> MSHPDYRMNLRPLGTPRGVSAVAGPHDIGASPGDKKSKNRSTRGKKKSIFETYMSKEDVSEGLKRGTLIQGVLRINPKKFHEAFIPSPDGDRDIFIDGVVARNRALNGDLVVVKLLPEEHWKVVKPESNDKETEAAYESDIPEELCGHHLPQQSLKSYNDSPDVIVEAQFDGSDSEDGHGITQNVLVDGVKKLSVCVSEKGREDGDAPVTKDETTCISQDTRALSEKSLQRSAKVVYILEKKHSRAATGFLKLLADKNSELFRKYALFSPSDHRVPRIYVPLKDCPQDFVARPKDYANTLFICRIVDWKEDCNFALGQLAKSLGQAGEIEPETEGILTEYGVDFSDFSSEVLECLPQGLPWTIPPEEFSKRRDLRKDCIFTIDPSTARDLDDALSCKPLADGNFKVGVHIADVSYFVPEGSDLDKVAAERATSVYLVQKVVPMLPRLLCEELCSLNPMSDKLTFSVIWTLTPEGKILDEWFGRTIIRSCTKLSYEHAQSMIESPTEKIPAKELPPISPEHSSEEVHQAVLNLHGIAKQLRQQRFVDGALRLDQLKLAFTLDHETGLPQGCHIYEYRESNKLVEEFMLLANMAVAHKIHRAFPEQALLRRHPPPQTRMLSDLVEFCDQMGLPVDFSSAGALNKSLTQTFGDDKYSLARKEVLTNMCSRPMQMALYFCSGLLQDPAQFRHYALNVPLYTHFTSPIRRFADVLVHRLLAAALGYRERLDMAPDTLQKQADHCNDRRMASKRVQELSTSLFFAVLVKESGPLESEAMVMGILKQAFDVLVLRYGVQKRIYCNALALRSHHFQKVGKKPELTLVWEPEDMEQEPAQQVITIFSLVEVVLQAESTALKYSAILKRPGTQGHLGPEKEEEESDGEPEDSSTS

Dis3-like 2 (Dis3L2) is a 3′–5′ exoribonuclease that plays a critical role in human development. Dis3L2 independently degrades structured substrates, including coding and noncoding 3′ uridylated RNAs. Unlike a number of structurally similar homologs, Dis3L2 can degrade structured RNAs independent of external helicase activity. We determined the structures of an RNase R/II family nuclease bound to a series of structured RNA substrates and analyzed the kinetic profiles of wild-type Homo sapiens Dis3L2 (HsDis3L2) and engineered mutants to reveal how this nuclease achieves highly efficient degradation of structured RNA.

To examine the structural changes occurring upon substrate processing, we shortened the 3′ overhang to 12 uridines and further modified the stem to increase stability (hairpinC–U12). We obtained a 3.1 Å structure of wild-type HsDis3L2 with hairpinC–U12 in which the double-helical stem of the RNA hairpin is clearly visible and nestled between the two CSDs and the S1 domain. The overall conformation of Dis3L2 does not change compared with the hairpinA–GCU14 or RNA-free Dis3L2 (RMSD = 0.56 and 0.61 Å, calculated over all Cα pairs, respectively). The basal junction of the hairpin interacts with the S1 and CSD1 domains, while the apical loop interacts with CSD2. At this point, when the 3′ overhang is 12 nucleotides long, the 5′ end at the double strand–single strand junction moves toward a loop in CSD1 (N76–H81). While the true start of the duplex (C2–G21) lies slightly closer to the S1 domain, the U1 5′ overhang forms a wobble base pair with U23 near the N76–H81 loop in CSD1. We observe a steeper decline in the koff starting around 11 nucleotides, which could reflect additional stabilizing interactions that become available when the phosphate backbone of the double-helical portion of the substrate is brought into contact with the enzyme (as was observed in the hairpinC–U12 and hairpinD–U7 structures). When the overhang is shortened to 11 or 12 nucleotides, the RNA duplex engages with the enzyme, stabilized by contacts with the S1 domain and CSDs.>[2x]QSITDYNYKKPLHNDYQILDKSKIFGSNSGSFVMYSMAADAYYIYNEKESRKRYSPNSTYKIYLAMFGLDRHIINDENSRMSWNHKHYPFDAWNKEQDLNTAMQNSVNWYFERISDQIPKNYTATQLKQLNYGNKNLGSY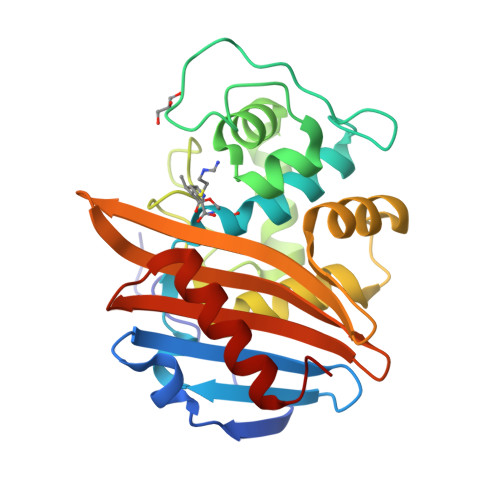KSYWMEDSLKISNLEQVIVFKNMMEQNNHFSKKAKNQLSSSLLIKKNEKYELYGKTGTGIVNGKYNNGWFVGYVITNHDKYYFATHLSDGKPSGKNAELISEKILKEMGVLN> QTARK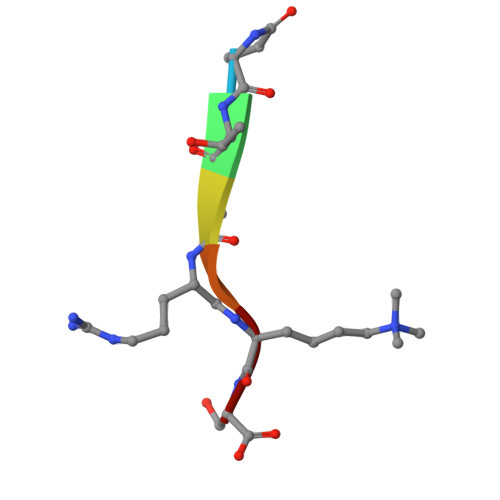S Oligosaccharyltransferase (OST) is the central enzyme of N-linked protein glycosylation. It catalyzes the transfer of a pre-assembled glycan, GlcNAc2Man9Glc3, from a dolichyl-pyrophosphate donor to acceptor sites in secretory proteins in the lumen of the endoplasmic reticulum. In higher metazoans and fungi, OST is a multimeric complex composed of eight subunits spatially arranged in three subcomplexes that are formed during OST assembly. Subcomplex I contains OST1 and OST5; subcomplex II contains OST3 (or OST6), STT3, and OST4; and subcomplex III contains OST2, WBP1, and SWP1.

We identified two distinct functional states of OST in this sample: A binary complex containing bound LLO (resolved at 3.0 Å resolution) and a ternary complex containing both donor and acceptor substrates (resolved at 3.1 Å resolution). In the structure containing Dol20-PP-GlcNAc2Man9Glc3, we observed well-defined EM density covering the catalytically important divalent ion Mn2+, the four isoprenyl units of Dol20, the pyrophosphate group, and the entire A-branch glycan, which includes two GlcNAc units at the reducing end, four mannose units, and the three terminal glucoses. The Dol20 lipid reaches approximately halfway across the membrane and is accommodated in a hydrophobic groove formed by TM6 and TM11 of the catalytic subunit STT3. The pyrophosphate group is coordinated by the manganese (II) ion and the STT3 residues Trp208 and Arg404. The A-branch of the glycan revealed a stretched or extended conformation, oriented parallel to the membrane plane, and is in contact with OST residues over its entire length. While all the nine hexose units of the A-branch were well defined in the EM density, we identified two regions where the glycan was specifically recognized: (1) the GlcNAc2 group at the reducing-end and (2) the terminal Glc3 moiety at the non-reducing end. Close to the active site, Tyr521 and Asn536 form hydrogen bonds with the N-acetyl group of the first GlcNAc, while Thr537 interacts with the second GlcNAc unit. At the non-reducing end, the terminal Glc3 are accommodated in a binding pocket formed by the auxiliary subunits OST2 and WBP1. Specifically, the terminal α,1-2 glucose interacts with Tyr383 of the WBP1 subunit via CH-π stacking, whereas the penultimate glucose interacts via hydrogen bonding with Asn75 of the OST2 subunit. Binding of LLO to an apo-state of OST leads to the formation of an “LLO-primed” state, where EL5 and TM9 remain unengaged and allowing access of a glycosylation sequon to the active site.

> MGSDRSCVLSVFQTILKLVIFVAIFGAAISSRLFAVIKFESIIHEFDPWFNYRATKYLVNNSFYKFLNWFDDRTWYPLGRVTGGTLYPGLMTTSAFIWHALRNWLGLPIDIRNVCVLFAPLFSGVTAWATYEFTKEIKDASAGLLAAGFIAIVPGYISRSVAGSYDNEAIAITLLMVTFMFWIKAQKTGSIMHATCAALFYFYMVSAWGGYVFITNLIPLHVFLLILMGRYSSKLYSAYTTWYAIGTVASMQIPFVGFLPIRSNDHMAALGVFGLIQIVAFGDFVKGQISTAKFKVIMMVSLFLILVLGVVGLSALTYMGLIAPWTGRFYSLWDTNYAKIHIPIIASVSEHQPVSWPAFFFDTHFLIWLFPAGVFLLFLDLKDEHVFVIAYSVLCSYFAGVMVRLMLTLTPVICVSAAVALSKIFDIYLDFKTSDRKYAIKPAALLAKLIVSGSFIFYLYLFVFHSTWVTRTAYSSPSVVLPSQTPDGKLALIDDFREAYYWLRMNSDEDSKVAAWWDYGYQIGGMADRTTLVDNNTWNNTHIAIVGKAMASPEEKSYEILKEHDVDYVLVIFGGLIGFGGDDINKFLWMIRISEGIWPEEIKERDFYTAEGEYRVDARASETMRNSLLYKMSYKDFPQLFNGGQATDRVRQQMITPLDVPPLDYFDEVFTSENWMVRIYQLKKDDAQGRTLRDVGELTRSSTKTRRSIKRPELGLRV;> MISDEQLNSLAITFGIVMMTLIVIYHAVDSTMSPKNRTLQVDGGSGGSLEVLFQGPTETSQVAPA;> MTYEQLYKEFHSSKSFQPFIHLDTQPKFAICGLIVTLAVLSSALFAVGSKSSYIKKLFFYTILSVIGSLFAGLTTVFASNSFGVYV;> MAKAPKANTPKVTSTSSAVLTDFQETFKTSKRAYFAQIEKYPKLKLIDTFCFFLVLLGVIQCTFIILIRDNFPFNAFLAGFIICVGQFVLLMSLRLQLCNSFPGISKNRAFAEFIVASLILHFVCLHFIN;> MRQVWFSWIVGLFLCFFNVSSAAQYEPPATWENVDYKRTIDVSNAYISETIEITIKNIASEPATEYFTAFESGIFSKVSFFSAYFTNEATFLNSQLLANSTTAPGDDGESEIRYGIIQFPNAISPQEEVSLVIKSFYNTVGIPYPEHVGMSEEQHLLWETNRLPLSAYDTKKASFTLIGSSSFEEYHPPNDESLLGKANGNSFEFGPWEDIPRFSSNETLAIVYSHNAPLNQVVNLRRDIWLSHWASTIQFEEYYELTNKAAKLSKGFSRLELMKQIQTQNMRQTHFVTVLDMLLPEGATDHYFTDLVGLVSTSHAERDHFFIRPRFPIFGGWNYNFTVGWTNKLSDFLHVSSGSDEKFVASIPILNGPPDTVYDNVELSVFLPEGAEIFDIDSPVPFTNVSIETQKSYFDLNKGHVKLTFSYRNLISQVANGQVLIKYDYPKSSFFKKPLSIACYIFTALMGVFVLKTLNMNVTN;> MQFFKTLAALVSCISFVLAYVAQDVHVSFPSTAGKSRVMIGKVEPRIGIDETVPTTITVEDPNEVIQVNFAIESTNKPFQNTLLIGLPNKNLEMAFEPEIKDNGKLSMYKYRIDLAKLDAALLQEASRSPEPIKATLILASSTAKPKENLFREILQLNLNFDVDHSDSSLVDKFGIKPEIHHIFHAEPKRVAKPIAVIFVLIIFITILSLIVTWLNSCAAAFNNIPTGVTAVYFLGFIATIVGFEVIFARYYLGTSIFETLFSSLYLGAPGLLTSTKFLRSFGTI;> MRTDWNFFFCILLQAIFVVGTQTSRTLVLYDQSTEPLEEYSVYLKDLEQRNYKLEYLDINSTSTTVDLYDKEQRLFDNIIVFPTKGGKNLARQIPVKQLIKFFENEGNILCMSSPGAVPNTIRLFLNELGIYPSPKGHVIRDYFSPSSEELVVSSNHLLNKYVYNARKSEDFVFGESSAALLENREQIVPILNAPRTSFTESKGKCNSWTSGSQGFLVVGFQNLNNARLVWIGSSDFLKNKNQDSNQEFAKELLKWTFNEKSVIKSVHAVHSHADGTSYDEEPYKIKDKVIYSVGFSEWNGEEWLPHIADDIQFELRQVDPYYRLTLSPSGNDSETQYYTTGEFILPDRHGVFTFLTDYRKIGLSFTTDKDVKAIRHLANDEYPRSWEISNSWVYISAICGVIVAWIFFVVSFVTTSSVGKKLETFKKTN;> MNWLFLVSLVFFCGVSTHPALAMSSNRLLKLANKSPKKIIPLKDSSFENILAPPHENAYIVALFTATAPEIGCSLCLELESEYDTIVASWFDDHPDAKSSNSDTSIFFTKVNLEDPSKTIPKAFQFFQLNNVPRLFIFKPNSPSILDHSVISISTDTGSERMKQIIQAIKQFSQVNDFSLHLPMDWTPIITSTIITFITVLLFKKQSKLMFSIISSRIIWATLSTFFIICMISAYMFNQIRNTQLAGVGPKGEVMYFLPNEFQHQFAIETQVMVLIYGTLAALVVVLVKGIQFLRSHLYPETKKAYFIDAILASFCALFIYVFFAALTTVFTIKSPAYPFPLLRLSAPFK>ANKPMQPITSTANKIVWSDPTRLSTTFSASL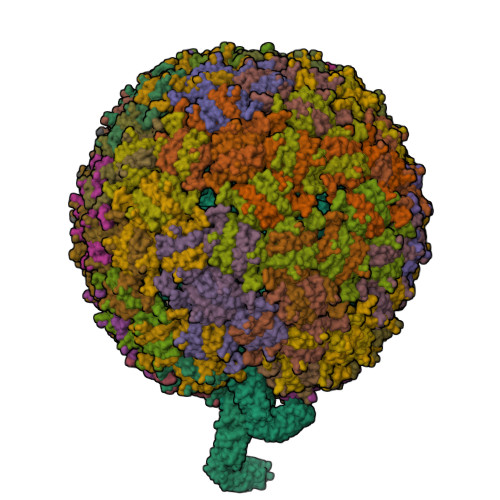LRQRVKVGIAELNNVSGQYVSVYKRPAPKPEGCADACVIMPNENQSIRTVISGSAENLATLKAEWETHKRNVDTLFASGNAGLGFLDPTAAIVSSDTT[178x];>[2x]MNMYKWVPESIRDSGEGQPSYSNNGDYAPSGPWVAAGIHTMPQSLRDSMRNSIMVTAQARRDVIGPEWGPDGRFTGYASVIGTPDPKPADIVNKFTVERRPVSNGNFQQRVKAGDIVVAPYTSDGKITVKLVAGQKDISSTPDYDYRIDSSLASSAGFVVAGERWYYTKRHFIIPRYFQNWRMRRRKYVTGWVMPTFYSPKEIFNRLKDSLVPDTGLVTQVWADNNTKRMDFLTAMAEIPQTLSSFLDALGYLGSLIKDFKRRRFFLNKAHQRIRNKLGVSFAERRSQIVSKYDRKIASARKPAIIVKLRQRKEKALKALDKMRVREEKKMIREFATQAASLWLSFRYEIMPLYYQSQDVLDVIANSTSEFMTSRDFVAKAINIGIPLEWNLDQENLVSQPRHNVMVKSKLSPENNIGKTLSVNPFTTAWELLTLSFVVDWFVNFGDVIAGFTGGYSDDSGATASWRFDDKKVFHLKNIPSAMVIVDINFYTRQVIDPRLCGGLAFSPKLNLFRYLDAMSLSWNRSRLKISRAT> MSAKEKFTSLSPAEFFKRNPELAGFPNPARALYQTVRELIENSLDATDVHGILPNIKITIDLIDDARQIYKVNVVDNGIGIPPQEVPNAFGRVLYSSKYVNRQTRGMYGLGVKAAVLYSQMHQDKPIEIETSPVNSKRIYTFKLKIDINKNEPIIVERGSVENTRGFHGTSVAISIPGDWPKAKSRIYEYIKRTYIITPYAEFIFKDPEGNVTYYPRLTNKIPKPPQEVKPHPYGVDREEIKILINNLKRDYTIKEFLVNEFQSIGDTTADKILELAGLKPNKKVKNLTEEEITRLVETFKKDEDFRSPSADSLSVIGEDLIELGLKKIFNPDFAASITRKPKAYQGHPFIVEAGVAFGGSIPVGEEPIVLRYANKIPLIYDEKSDVIWKVVEELDWKRYGIESDQYQMVVMVHLCSTKIPYKSAGKESIAEVENIEKEIKNALMEVARKLKQYLSEKRKEQEAKKKLLAYLKYIPEVSRSLATFLASGNKEL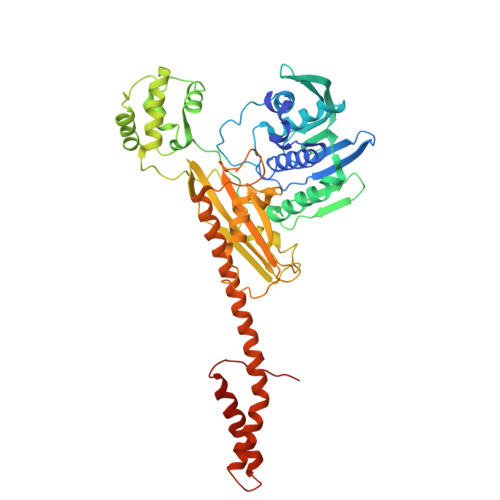VSKYQNEISEGLFKLISKKLDLINIEEYRKVYRVDSE> MGPKVQTDPPSVPICDLYPNGVFPKGQECEYPPTQDGRTAAWRTTSEEKKALDQASEEIWNDFREAAEAHRQVRKYVMSWIKPGMTMIEICEKLEDCSRKLIKENGLNAGLAFPTGCSLNNCAAHYTPNAGDTTVLQYDDICKIDFGTHISGRIIDCAFTVTFNPKYDTLLKAVKDATNTGIKCAGIDVRLCDVGEAIQEVMESYEVEIDGKTYQVKPIRNLNGHSIGQYRIHAGKTVPIVKGGEATRMEEGEVYAIETFGSTGKGVVHDDMECSHYMKNFDVGHVPIRLPRTKHLLNVINENFGTLA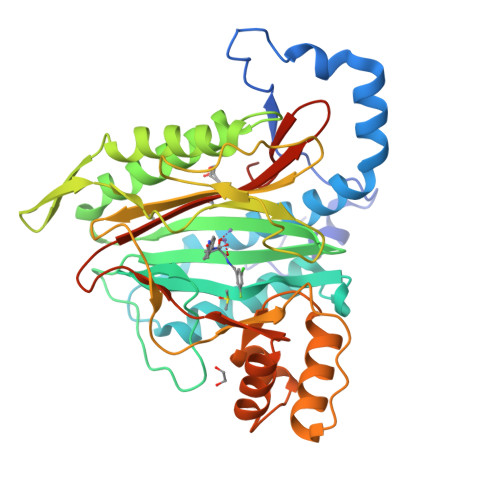FCRRWLDRLGESKYLMALKNLCDLGIVDPYPPLCDIKGSYTAQFEHTILLRPTCKEVVSRGDDYHHHHHH> IIGGREVIPHSRPYMASLQRNGSHLCGGVLVHPKWVLTAAHCLAQRMAQLRLVLGLHTLDSPGLTFHIKAAIQHPRYKPVPALENDLALLQLDGKVKPSRTIRPLALPSKRQVVAAGTRCSMAGWGLTHQGGRLSRVLRELDLQVLDTRMCNNSRFWNGSLSPSMVCLAADSKDQAPCKGDSGG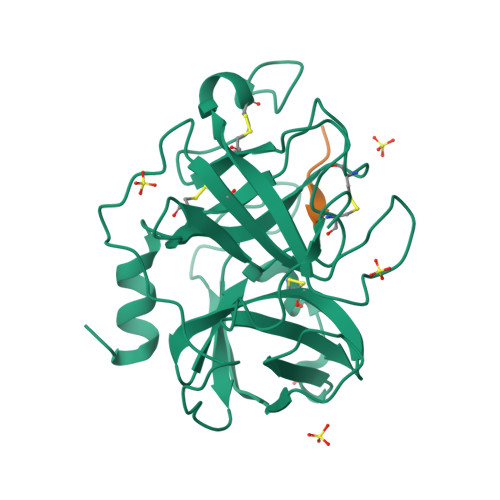PLVCGKGRVLAGVLSFSSRVCTDIFKPPVATAVAPYVSWIRKVTGRSALEHHHHHH;> SSGKVPL>MNRLPSSASALACSAHALNLIEKRTLDHEEMKALNREVIEYFKEHVNPGFLEYRKSVTAGGDYGAVEWQAGSLNTLVDTQGQEFIDCLGGFGIFNVGHRNPVVVSAVQNQLAKQPLHSQELLDPLRAMLAKTLAALTPGKLKYSFFCNSGTESVEAALKLAKAYQSPRGKFTFIATSGAFHGKSLGALSATAKSTFRKPFMPLLPGFRHVPFGNIEAMRTALNECKKTGDDVAAVILEPIQGEGGVILPPPGYLTAVRKLCDEFGALMILDEVQTGMGRTGKMFACEHENVQPDILCLAKALGGGVMPIGATIATEEVFSVLFDNPFLHTTTFGGNPLACAAALATINVLLEQNLPAQAEQKGDMLLDGFRQLAREYPDLVQEARGKGMLMAIEFVDNEIGYNFASEMFRQRVLVAGTLNNAKTIRIEPPLTLTIEQCELVIKAARKALAAMRVSVEEALEHHHHHH[4x]

YgjG is a putrescine aminotransferase (PATase, EC 2.6.1.82). Based on its amino acid sequence alignment, it belongs to the class III pyrodoxal-5′-phosphate (PLP)-dependent aminotransferase family, which include ornithine aminotransferase (OAT) and GABA aminotransferase (GABA-AT). In this study, we determined the crystal structures of YgjG from E. coli in free and putrescine-bound states at 2.3 and 2.1 Å resolutions, respectively, to investigate the structural basis of YgjG substrate specificity. The monomer comprises an N-terminal domain, a large PLP-binding domain, and a C-terminal domain.

The native YgjG crystal structure was determined at the resolution 2.3 Å through molecular replacement and refined to the Rwork and Rfree factors 18.1% and 23.3%, respectively. The crystallographic asymmetric unit contained four YgjG molecules that formed two dimers. The dimer formed extensive contacts between the two subunits. The buried surface area between the two subunits was 6,167 Å2, which corresponds to 30.2% of the total solvent accessible area. The YgjG active site is at the dimeric interface and includes the residues from both subunits. The cofactor PLP is located at the bottom of the active site and is involved in multiple interactions. The electron density for the cofactor clearly shows that PLP is covalently linked to the strictly conserved lysine residue (Lys300) via a Schiff base linkage. The PLP phosphate group interacts with four water molecules, Thr151, Gly150 and Thr332* (the asterisk indicating the other subunit) through hydrogen bonds. Similar to other class III aminotransferases, the Asp271 side chain is hydrogen bonded to the cofactor pyridine nitrogen. The PLP pyridine ring is sandwiched between the Phe180 and Val273 side chains.> MLEANVYDNFNPNYYNISDFSMPNGKKEKRGLPIPKARCQVINYELWETGYLYTSSATLTVSVEVGDIVQILFPEVVPIEEALGKKKKLNLDMVYLVTDVDESNKATLKNYFWAMIESLDVPNAITKTTNFAIIDYLIDPNKNNLMSYGYFFNSSIFAGKATINRKAETSSAHDVAKRIFSKVQFQPTTTIQHAPSETDPRNLLFINFASRNWNRKRITTRVDIK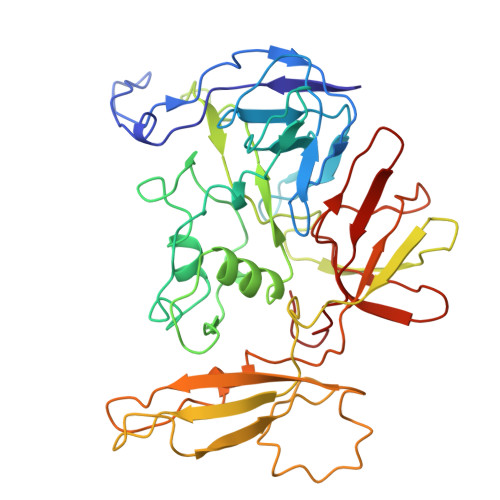QSVTMDTETIVERSAYNFAVVFVKNKATDDYTDPPKMYIAKNNGDVIDYSTYHGDGTDLPDVRTAKTLFYDRDDHGNPPELSTIKVEISPSTIVTRLIFNQNELLPLYVNDLVDIWYEGKLYSGYIADRVKTEFNDRLIFVESGDKPNVI>[2x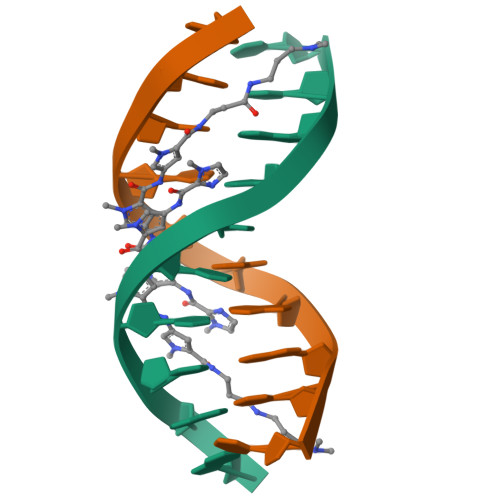]CCAGATCTGG> MTTTTATTAPEAALGVLPRADGSARYSHAGYTVTASVNGPIEAQRRDEHPYEAHVDVIVRPAAGVGGTRERHLESILQSSFAQIILVKSFPRSLIQIVLQVEESPENEYVNTK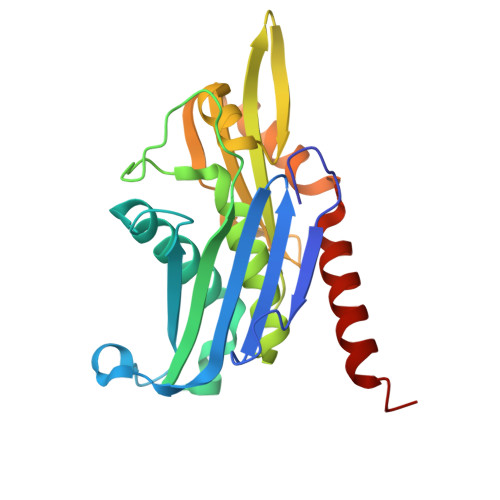LVQASLNFAVMPALFQTAMLALLSAGVPMRATATATAIALASENGATKTLIDPSPRQVELAQSVHVFAFTSQDELLLAESEGDFTIKEWDAAYETAKNICCRPSPTMDGVQMMAIDDDRLVGPDLRHFIRSTMEAKVATDLHWKS>MKVEEILEKALELVIPDEEEVRKGREAEEELRRRLDELGVEYVFVGSYARNTWLKGSLEIDVFLLFPEEFSKEELRERGLEIGKAVLDSYEIRYAEHPYVHGVVKGVEVDVVPCYKLKEPKNIKSAVDRTPFHHKWLEGRIKGKENEVRLLKGFLKANGIYGAEYKVRGFSGYLCELLIVFYGSFLETVKNARRWTRRTVIDVAKGEVRKGEEFFVVDPVDEKRNVAANLSLDNLARFVHLCREFMEAPSLGFFKPKHPLEIEPERLRKIVEERGTAVFAVKFRKPDIVDDNLYP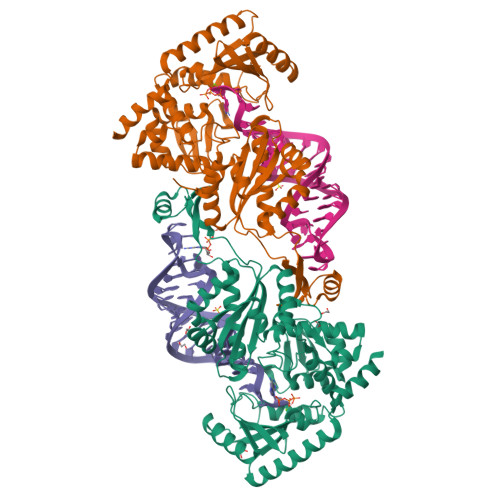QLERASRKIFEFLERENFMPLRSAFKASEEFCYLLFECQIKEISRVFRRMGPQFEDERNVKKFLSRNRAFRPFIENGRWWAFEMRKFTTPEEGVRSYASTHWHTLGKNVGESIREYFEIISGEKLFKEPVTAELCEMMGVKDCCCQ[2x]> MITLRKLIGNINMTKEPEQQSPLELWFERIIDVPLEKLTVEDLCRAIRQNLCIDQLMPRVLEVLTKEPLAGEYYDGELIAALSTIKGEDLKDQKST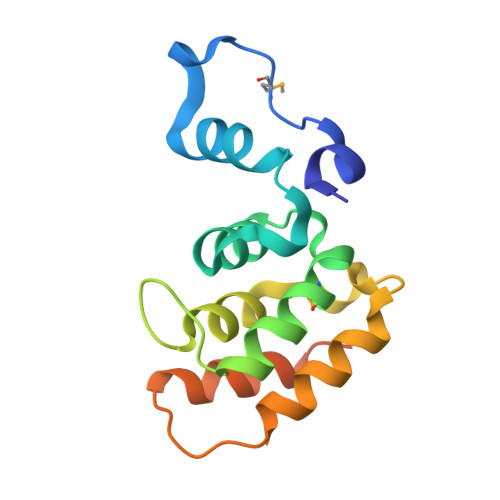FTQIRQLINQLEPSDINDDLRKDILKINQIIVTSLEHHHHHH(5R,10S,13R,14R,17R)-17-((R,E)-7-hydroxy-6-methylhept-5-en-2-yl)-4,4,10,13,14-pentamethyl-1,2,5,6,10,11,12,13,14,15,16,17-dodecahydro-3H-cyclopenta[a]phenanthrene-3,7(4H)-dione 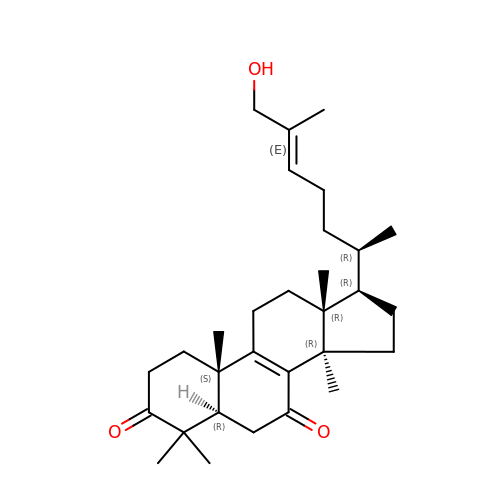| C30 H46 O3 | SDAWCNCFVWQZDP-GOUGDUPLSA-N>AGSSLQETEEVAVANEMSEAGSVDTDRFNVPLQKEKKRQSPREKQKRVMNTEKTGIAIIAPGGYVPDSDLQRAIGVLKSRGYEVFNYVDPQKRHERFAANDEERSRQIMEAATNPDVKIVIALRGGYGTTRLLHDLDFAKLAKSGKLFVGHSDFTVFEMALLKHGAVSFSGPMIQSDFTRGDLSAFTLNHFDETMTSPETSVKWVSKDNPDVDVEGTLWGGNLTMLAHMAGTPWMPDISGGILFVEDIHEHPYRVERMLLQLDESGILKKQKALVLGHFSEFKLSDYDNGYDFNAMLSWLRSRLSIPV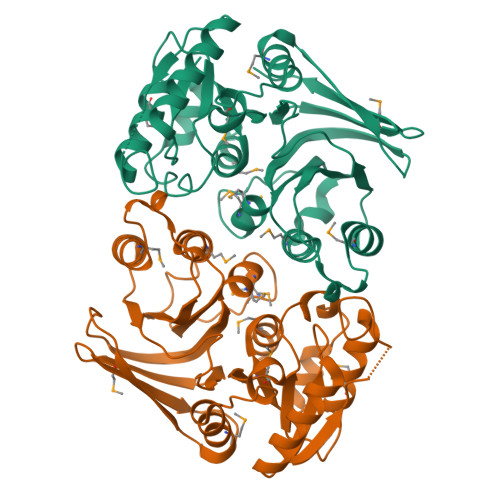VTGLPFGHTKDKVTLPVGGRAHLMSKAGKIQLDIGDYPTVR[2x]>MKVGIVGSGMVGSATAYALALLGVAREVVLVDLDRKLAQAHAEDILHATPFAHPVWVRAGSYGDLEGARAVVLAAGVAQRPGETRLQLLDRNAQVFAQVVPRVLEAAPEAVLLVATNPVDVMTQVAYRLSGLPPGRVVGSGTILDTARFRALLAEYLRVAPQSVHAY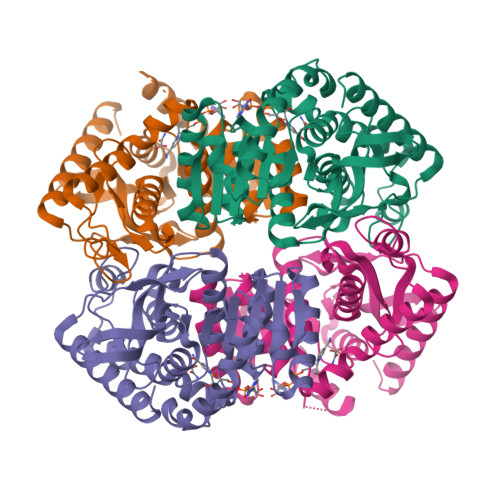VLGEHGDSEVLVWSSAQVGGVPLLEFAEARGRALSPEDRARIDEGVRRAAYRIIEGKGATYYGIGAGLARLVRAILTDEKGVYTVSAFTPEVEGVLEVSLSLPRILGAGGVEGTVYPSLSPEEREALRRSAEILKEAAFALGF[4x]>[2x]MNVFNPAQFRAQFPALQDAGVYLDSAATALKPEAVVEATQQFYSLSAGNVHRSQFAEAQRLTARYEAAREKVAQLLNAPDDKTIVWTRGTTESINMVAQCYARPRLQPGDEIIVSVAEHHANLVPWLMVAQQTGAKVVKLPLNAQRLPDVDLLPELITPRSRILALGQMSNVTGGCPDLARAITFAHSAGMVVMVDGAQGAVHFPADVQQLDIDFYAFSGHKLYGPTGIGVLYGKSELLEAMSPWLGGGK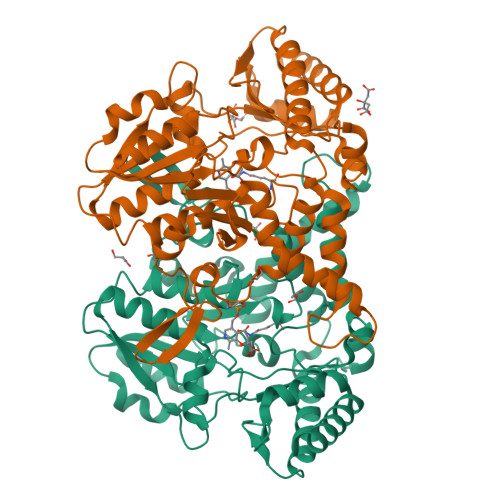MVHEVSFDGFTTQSAPWKLEAGTPNVAGVIGLSAALEWLADYDINQAESWSRSLATLAEDALAKRPGFRSFRCQDSSLLAFDFAGVHHSDMVTLLAEYGIALRAGQHCAQPLLAELGVTGTLRASFAPYNTKSDVDALVNAVDRALELLVD>TLRRRYTMVHQESLPNSTANSVDRQVGYFADNGVGNPLAIVQHPAGIHKNGITYVSYQGPKEDPYIASYNHQTGQWQGPFRAGISELGRRDGGKKFDNNGKPTMLIDDEGYIHIFYGGHGGQASNGKNPLGNTHHGANKHAVSKRPYDISQWEDLNNITPFGTYNQAIKMDNGDIYLFFRHGAHRSDWVYQKSVDNGRTFASPVSFLKHKRRTDIDAVDSWYAWAGKGQGDNIIVSYDYHVCWDGGAGVNGRGHTTERHDVYFMSFNTKTGEWSNVEGEKLVLPVTREVADEKTMAMRTGELWTFNGSTHLDAQGQPHIAINAGIDKGAKTGGPKQTRHVRWNGNEWVGGDKVIPQYERVSRGDFMVTDPENIRYLTTYNQDNDAVLSWWQSHDGGEHFVEDKTVLRKDNASFAISAFIKDAIPDAQMLVAEKVSDEGIKMYLVGEEGAVTRSLVDLKTAMPTSKLEHHHHH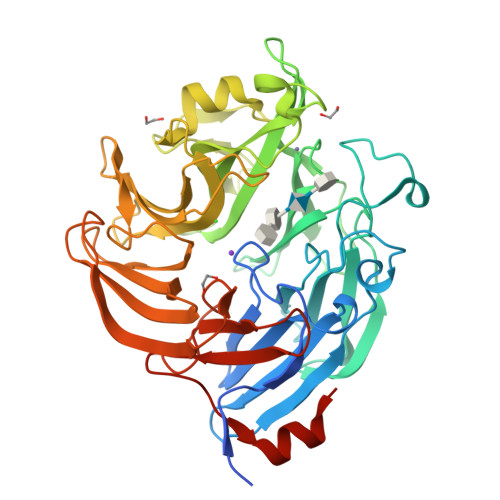H[2x]>MIDQTALATEIKRLIKAAGPMPVWRYMELCLGHPEHGYYVTRDPLGREGDFTTSPEISQMFGELLGLWSASVWKAADEPQTLRLIEIGPGRGTMMADALRALRVLPILYQSLSVHLVEINPVLRQKQQTLLAGIRNIHWHDSFEDVPEGPAVILANEYFDVLPIHQAIKRETGWHERVIEIGASGELVFGVAADPIPGFEALLPPLARLSPPGAVFEWRPDTEILKIASRVRDQGGAALIIDYGHLRSDVGDTFQAIASHSYADPLQHPGRADLTAHVDFDALGRAAESIGARAHGPVTQGA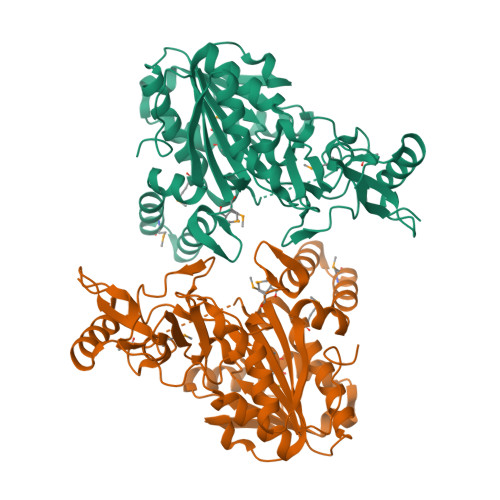FLKRLGIETRALSLMAKATPQVSEDIAGALQRLTGEGRGAMGSMFKVIGVSDPKIETLVALSDDTDREAERRQGTHGLEHHHHHH[2x]>[2x]MKTIIINGVQFNTDEDTTILKFARDNNIDISALCFLNNCNNDINKCEICTVEVEGTGLVTACDTLIEDGMIINTNSDAVNEKIKSRISQLLDIHEFKCGPCNRRENCEFLKLVIKYKARASKPFLPKDKTEYVDERSKSLTVDRTKCLLCGRCVNACGKNTETYAMKFLNKNGKTIIGAEDEKCFDDTNCLLCGQCIIACPVAALSEKSHMDRVKNALNAPEKHVIVAMAPSVRASIGELFNMGFGVDVTGKIYTALRQLGFDKIFDINFGADMTIMEQATELVQRIENNGPFPMFTSCCPGWVRQAENYYPELLNNLSSAKSPQQIFGTASKTYYPSISGLDPKNVFTV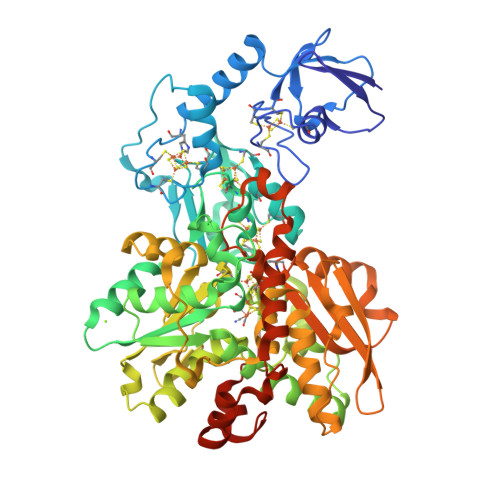TVMPCTSKKFEADRPQMEKDGLRDIDAVITTRELAKMIKDAKIPFAKLEDSEADPAMGEYSGAGAIFGATGGVMEAALRSAKDFAENAELEDIEYKQVRGLNGIKEAEVEINNNKYNVAVINGASNLFKFMKSGMINEKQYHFIEVMACHGGCVNGGGQPHVNPKDLEKVDIKKVRASVLYNQDEHLSKRKSHENTALVKMYQNYFGKPGEGRAHEILHFKYKKSAWSHPQFEK>[2x]MAYRKRGARREANINNNDRMQEKDDEKQDQNNRMQLSDKVLSKKEEVVTDSQEEIKIADEVKKSTKEESKQLLEVLKTKEEHQKEIQYEILQKTIPTFEPKESILKKLEDIKPEQAKKQTKLFRIFEPRQLPIYRANGEKELRNRWYWKLKKDTLPDGDYDVREYFLNLYDQVLTEMPDYLLLKDMAVENKNSRDAGKVVDSETASICDAIFQDEETEGAVRRFIAEMRQRVQADRNVVNYPSILHPIDYAFNEYFLQHQLVEPLNNDIIFNYIPERIRNDVNYILNMDRNLPSTARYIRPNLLQDRLNLHDNFESLWDTITTSNYILARSVVPDLKELVSTEAQIQKMSQDLQLEALTIQSETQFLTGINSQAANDCFKTLIAAMLSQRTMSLDFVTTNYMSLISGMWLLTVVPNDMFIRESLVACQLAIVNTIIYPAFGMQRMHYRNGDPQTPFQIAEQQIQNFQVANWLHFVNNNQFRQVVIDGVLNQVLNDNIRNGHVINQLMEALMQLSRQQFPTMPVDYKRSIQRGILLLSNRLGQLVDLTRLLAYNYETLMACVTMNMQHVQTLTTEKLQLTSVTSLCMLIGNATVIPSPQTLFHYYNVNVNFHSNYNERINDAVAIITAANRLNLYQKKMKAIVEDFLKRLHIFDVARVPDDQMYRLRDRLRLLPVEVRRLDIFNLILMNMDQIERASDKIAQGVIIAYRDMQLERDEMYGYVNIARNLDGFQQINLEELMRTGDYAQITNMLLNNQPVALVGALPFVTDSSVISLIAKLDATVFAQIVKLRKVDTLKPILYKINSDSNDFYLVANYDWVPTSTTKVYKQVPQQFDFRNSMHMLTSNLTFTVYSDLLAFVSADTVEPINAVAFDNMRIMNEL;>[13x]MDVLYSLSKTLKDARDKIVEGTLYSNVSDLIQQFNQMIITMNGNEFQTGGIGNLPIRNWNFDFGLLGTTLLNLDANYVETARNTIDYFVDFVDNVCMDEMVRESQRNGIAPQSDSLRKLSGLKFKRINFDNSSEYIENWNLQNRRQRTGFTFHKPNIFPYSASFTLNRSQPAHDNLMGTMWLNAGSEIQVAGFDYSCAINAPANTQQFEHIVQLRRVLTTATITLLPDAERFSFPRVINSADGATTWYFNPVILRPNNVEVEFLLNGQIINTYQARFGTIIARNFDTIRLSFQLMRP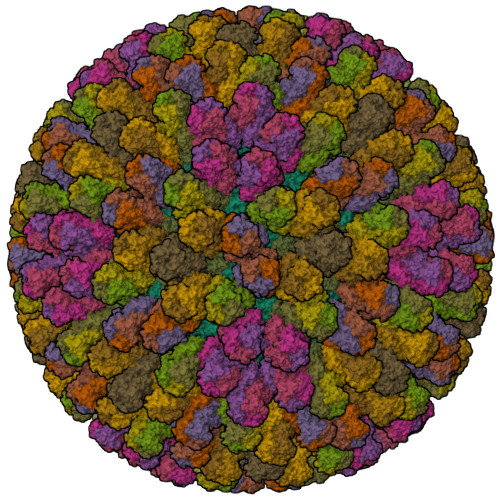PNMTPAVAALFPNAQPFEHHATVGLTLRIESAVCESVLADASETMLANVTSVRQEYAIPVGPVFPPGMNWTDLITNYSPSREDNLQRVFTVASIRSMLVK;> MGKYNLILSEYLSFIYNSQSAVQIPIYYSSNSELENRCIEFHSKCLENSKNGLSLRKLFVEYNDVIENATLLSILSYSYDKYNAVERKLVKYAKGKPLEADLTVNELDYENNKMTSELFPTAEEYTDSLMDPAILTSLSSNLNAVMFWLEKHENDVAEKLKVYKRRLDLFTIVASTINKYGVPRHNAKYRYEYDVMKDKPYYLVTWANSSIEMLMSVFSHDDYLIAKELIVLSYSNRSTLAKLVSSPMSILVALVDINGTFITNEELELEFSNKYVRAIVPDQTFDELNQMLDNMRKAGLVDIPKMIQDWLVDRSIEKFPLMAKIYSWSFHVGFRKQKMLDAALDQLKTEYTENVDDEMYREYTMLIRDEVVKMLEEPVKHDDHLLRDSELAGLLSMSSASNGESRQLKFGRKTIFSTKKNMHVMDDMANERYTPGIIPPVNVDKPIPLGRRDVPGRRTRIIFILPYEYFIAQHAVVEKMLIYAKHTREYAEFYSQSNQLLSYGDVTRFLSNNTMVLYTDVSQWDSSQHNTQPFRKGIIMGLDILANMTNDAKVLQTLNLYKQTQINLMDSYVQIPDGNVIKKIQYGAVASGEKQTKAANSIANLALIKTVLSRISNKHSFATKIIRVDGDDNYAVLQFNTEVTKQMIQDVSNDVRETYARMNAKVKALVSTVGIEIAKRYIAGGKIFFRAGINLLNNEKRGQSTQWDQAAILYSNYIVNRLRGFETDREFILTKIMQMTSVAITGSLRLFPSERVLTTNSTFKVFDSEDFIIEYGTTVDEVYIQRAFMSLSSQKSGIADEIAASSTFKNYVTRLSEQLLFSKNNIVSRGIALTEKAKLNSYAPISLEKRRAQISALLTMLQKPVTFKSSKITINDILRDIKPFFTVSDAHLPIQYQKFMPTLPDNVQYIIQCIGSRTYQIEDDGSKSAISRLISKYSVYKPSIEELYKVISLHENEIQLYLISLGIPKIDADTYVGSKIYSRDKYRILESYVYNLLSINYGCYQLFDFNSPDLEKLIRIPFKGKIPAVTFILHLYAKLEVINYAIKNGSWISLFCNYPKSEMIKLWKKMWNITSLRSPYTNANFFQEP> MAQKTFKVTADSGIHARPATVLVQTASKYDADVNLEYNGKTVNLKSIMGV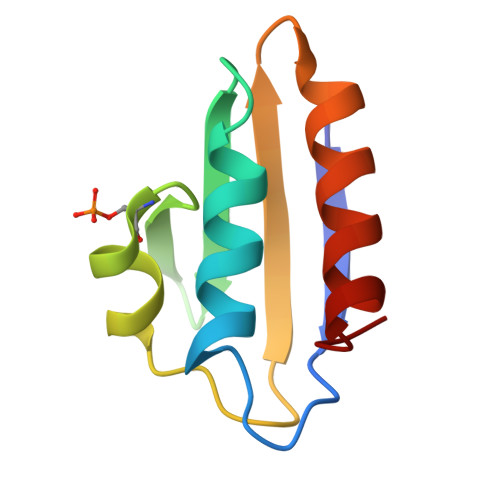MSLGIAKGAEITISASGADENDALNALEETMKSEGLGE> MRTFFVGGNWKANPKTVQEAEKLVEMLNGAKVEGNVEVVVAAPFVFLPTLQQKLRKDWKVSAENVFTKPNGTVPMIKSFGIEWTILGHSERRDILKEDDEFL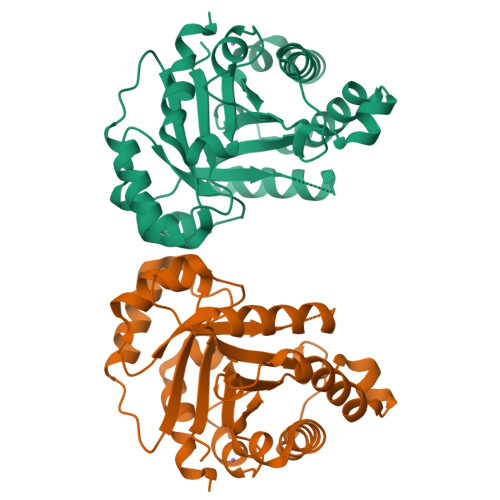AAKAKFALENGMKIIYCCGEHLSEREAGKASEFVSAQIEKMIPAIPAGKWDDVVIAYEPIWAIGTGKVASTQDAQEMCKVIRDILAAKVGADIANKVRILYGGSVKPNNCNELAACPDVDGFLVGGASLEAGFINIVNSNVHSK>[2x]DSTTQTTEQSKKNNDKPQDVITTSEIRKLNEKEPVYIYTSAAGGGFHMIPRTARLCTILTANRIPFTYRDLGTDDEARKVWKTFSKGRSLPGVVRGH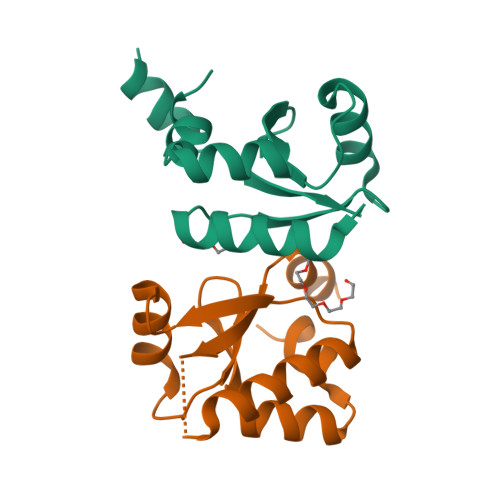NDLIGNWEEIEEANEDYKLRELIYDTI Safe iron storage, detoxification and appropriate delivery of iron for biosynthetic functions in a cell are carried out by a superfamily of proteins known as ferritins that are widely found in all domains of life. A subfamily of ferritin superfamily found in eubacteria, called bacterioferritins (Bfrs), differ from ferritins in having additional noncovalently bound haem groups. The Mtb genome reveals the presence of two putative iron-storage proteins, namely, BfrA (Rv1876)–a bacterioferritin and BfrB (Rv3841)–a ferritin like protein. The structure of Mtb SeMet-BfrA exhibits the highly conserved architecture of ferritin superfamily where the complete biological molecule is assembled into an almost spherical shell by the symmetrical association of 24 equivalent monomers that are related by operation of 4-, 3- and 2-fold symmetry axes.

We have determined the crystal structure of selenomethionyl analog of bacterioferritin A (SeMet-BfrA) from M. tuberculosis and carried out in-depth analysis to identify sub regions of structure unique to Mycobacterium species. The crystal structure of Mtb SeMet-BfrA has been determined by Molecular Replacement (MR) using the structure of the recently published M. smegmatis BfrA as template and refined to a final Rwork value of 19% and an Rfree value of 23% at 2.5 Å resolution. The crystal structure of SeMet-BfrA additionally demonstrates that SeMet incorporation changes the electronic environment in the haem-binding pocket of the protein leading to demetallation and cleavage of haem ligand. Moreover, the circumference of the horse-shoe shaped electron density ring appearing at the documented haem position in the SeMet-BfrA structure was larger than expected for the haem porphyrin ring and appeared broken between two five-membered pyrroles strongly suggesting the presence of a metal-free and degraded porphyrin derivative. On further exploring the shape of the electron density, the break in the density advocated that the porphyrin ring is cleaved at its γ-meso carbon position, resulting probabaly in the generation of biliverdin IX-γ isomer as the main end product. Moreover, since the mass spectrometry analysis of Mtb native and SeMet-BfrA crystals was unable to provide a clear evidence about the presence of biliverdin as the haem degradation product, this ligand has been designated as ‘unknown ligand’ (UNL) in the deposited PDB. The best temperature factors and Rfree value were obtained when iron was refined with 0.3 occupancy in both Fe1 and Fe2 sites. A close examination of the di-iron site in our crystal structure reveals that this structure is compatible with the reduced form of bacterioferritin. A pore, termed the B-site, is large enough to accommodate an iron atom and is lined mostly with negatively charged residues Asn34, Asp66, Asp132, Glu135, Thr136 and Glu139 and hence maybe the most likely route for iron entry/exit to/from the Bfr cavity.

>ASGSMQGDPDVLRLLNEQLTSELTAINQYFLHSKMQDNWGFTELAAHTRAESFDEMRHAEEITDRILLLDGLPNYQRIGSLRIGQTLREQFEADLAIEYDVLNRLKPGIVMCREKQDTTSAVLLEKIVADEEEHIDYLETQLELMDKLGEELYSAQCVSRPPTSAWSHPQFEK[6x]>[4x]GSIINETADDIVYRLTVIIDDRYESLKNLITLRADRLEMIINDNVSTILASI

RHCC-NT was first described as an S-layer protein component of the archaea Staphylothermus marinus. Here, we present an unconventional drug delivery device entitled Right-Handed Coiled Coil-Nanotube (RHCC-NT) which is ideally suited to uptake boron clusters into its large internal cavities. In addition to binding small molecules, this nanotube can be internalized by eukaryotic cells, which offers possibilities for targeted drug delivery in BNCT. Although the polydispersity of the sample increased, the cumulant radius remained the same over the temperature gradient. This highly stable tetrameric structure prevents the protein from dissociating or exposing the hydrophobic cavities to the exterior.

Carborane, C2B10H12, a boron rich compound with applications in Boron Neutron Capture Therapy, binds into the hydrophobic cavities of RHCC-NT upon mutual incubation at 50 °C. We observed that the chemical interactions that stabilize the o-carborane inside the cavity are mainly hydrophobic, mediated by the amino acid side chains of Leu and Ile of the respective cavity. Based on spatial analysis, the two center cavities each have a spherical volume of around 240 Å3, allowing for binding of the o-carborane clusters with their steric bulk of 148 Å334. The outer cavities have a spatial volume of around 180 Å3, surrounded by hydrophobic amino acid side chains which would also allow for o-carborane ligand binding. Nonetheless, based on experimental electron densities, we detected that three out of the four nanotube cavities contain boron clusters; o-carborane is absent in the N-terminal cavity of the nanotube. Thus, ligand incubation allows for an integration of 30 boron atoms per nanotube. Interestingly, the uptake of o-carborane did not cause any final conformational changes to the nanotube which is most likely due to the extreme rigidity of the macromolecule caused by its many intramolecular interactions such as salt bridges and additional hydrophobic interactions between the helices. Thus, transfer of o-carborane into the hydrophobic cavities and displacement of the water clusters is energetically favourable due to the hydrophobic effect. The nanotube has a length of approximately 7.7 nm and a diameter of 1.8 nm, binding three o-carborane molecules.>[2x]GPLGSDFPQHSQHVLEQLNQQRQLGLLCDCTFVVDGVHFKAHKAVLAACSEYFKMLFVDQKDVVHLDISNAAGLGQVLEFMYTAKLSLSPENVDDVLAVATFLQMQDIITACHALKSLARSGGGSSGGSGTAQTLQMEIPNFGNSILECLNEQRLQGLYCDVSVVVKGHAFKAHRAVLAASSSYFRDLFNNSRSAVVELPAAVQPQSFQQILSFCYT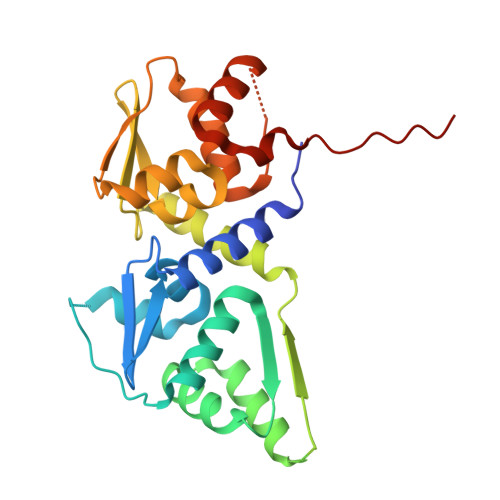GRLSMNVGDQDLLMYTAGFLQIQEIMEKGTEFFLKVSS> PHMQPFDSGHDDLVHDVVYDFYGRHVATCSSDQHIKVFKLDKDTSNWELSDSWRAHDSSIVAIDWASPEYGRIIASASYDKTVKLWEEDPDQEECSGRRWNKLCTLNDSKGSLYSVKFAPAHLGLKLACLGNDGILRLYDALEPSDLRSWTLTSEMKVLSIPPANHLQSDFCLSWCPSRFSPEKLAVSALEQAIIYQRGKDGKLHVAAKLPGHKSLIRSISWAPSIGRWYQLIATGCKDGRIRIFKI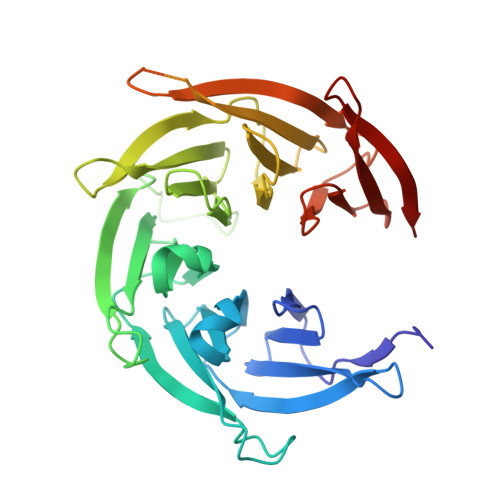TEKLSPLASEESLTNSNMFDNSADVDMDAQGRSDSNTEEKAELQSNLQVELLSEHDDHNGEVWSVSWNLTGTILSSAGDDGKVRLWKATYSNEFKCMSVITAQQ Tyrosinases form an ubiquitous family of metalloenzymes and are found in all domains of life. Tyrosinases catalyze the ortho-hydroxylation of monophenols to o-diphenols (monophenolase or cresolase activity, EC 1.14.18.1) as well as the subsequent two-electron oxidation to the respective o-quinones (diphenolase or catechol oxidase activity, EC 1.10.3.1), which is coupled with the reduction of molecular oxygen to water. Activation of molecular oxygen is affected by binding of dioxygen to the type III copper center in a characteristic ‘side-on’ bridging mode (µ-η2:η2). The purity of these preparations is further compromised by the fact that Agaricus bisporus possesses genes coding for six different tyrosinases (AbPPO1 - AbPPO6).

Herein, we describe such a protocol, yielding pure AbPPO4 in its latent form as well as providing access to the mature, active form of the enzyme. Here, the latent form of AbPPO4 is produced by E. coli at a yield of 110 to 140 mg per liter of culture. ESI-MS of the acidified (causes the loss of copper)27 but otherwise intact protein yielded a mass of 65096.7 ± 0.30 Da for the latent tyrosinase which matches the calculated mass of 65096.46 Da for the complete sequence from the N-terminal glycine at position −8 to the C-terminal threonine 565 with one thioether bridge (−2.016 Da) and one closed disulfide bridge (−2.016 Da). Latent tyrosinase crystallized in the monoclinic space group C 1 2 1 with 4 chains in the asymmetric unit giving rise to a unit cell of a = 287.30 Å, b = 52.09 Å, c = 152.66 Å, α = 90.00°, β = 98.03° and γ = 90.00°. The obtained crystals diffracted to a resolution of 3.25 Å (for further statistics see Table S2). In contrast to the crystals obtained with the enzyme isolated from the natural source which contained two different chains in the asymmetric unit (one latent and one active protein)33 and did only form in the presence of sodium hexatungstotellurate(VI) (Na6[TeW6O24] • 22 H2O, TEW), the recombinant enzyme formed crystals containing exclusively the latent tyrosinase. Inspection of the electron density gave no indication for any deviation from the sequence shown in Fig. 5. The amino acid side chains which form hydrogen bonds with the TEW polyoxyanion in the crystal of the enzyme purified from the natural source (HKKE starting at H116) are found in equivalent positions in the crystal of the recombinant enzyme but the lysine side chains are considerably more flexible as indicated by the lack of electron density beyond the Cβ-atoms.

>[4x]GPLGSPGIPMSLLATVGPTGGVKNRLDIVDFVRDEKFFTLYVRALQAIQDKDQADYSSFFQLSGIHGLPFTPWAKPKDTPTVPYESGYCTHSQVLFPTWHRVYVSIYEQVLQEAAKGIAKKFTVHKKEWAQAAEDLRQPYWDTGFALVPPDEIIKLEQVKITNYDGTKITVRNPILRYSFHPIDPSFNGYPNFDTWRTTVRNPDADKKENIPALIAKLDLEADSTREKTYNMLKFNANWEAFSNHGEFDDTHANSLEAVHDDIHGFVGRGAIRGHMTHALFAAFDPIFWLHHSNVDRHLSLWQALYPGVWVTQGPEREGSMGFAPGTELNKDSALEPFYETEDKPWTSVPLTDTALLNYSYPDFDKVKGGTPDLVRDYINDHIDRRYGIKKSEGGKNPALDLLSDFKGVTHDHNEDLKMFDWTIQASWKKFELDDSFAIIFYFAADGSTNVTKENYIGSINIFRGTTPTNCANCRTQDNLVQEGFVHLDRFIARDLDTFDPQAVHRYLKEKKLSYKVVADDHSVTLKSLRIRVQGRPLHLPPGVSFPRLDKNIPIVNFDDVLDLVTGVVNIGLT(5~{S},6~{E},8~{S},9~{S},12~{R},15~{E})-21-chloranyl-12,20-dimethoxy-6,8,16-trimethyl-5,9-bis(oxidanyl)-2-azabicyclo[16.3.1]docosa-1(21),6,15,18(22),19-pentaene-3,11-dione 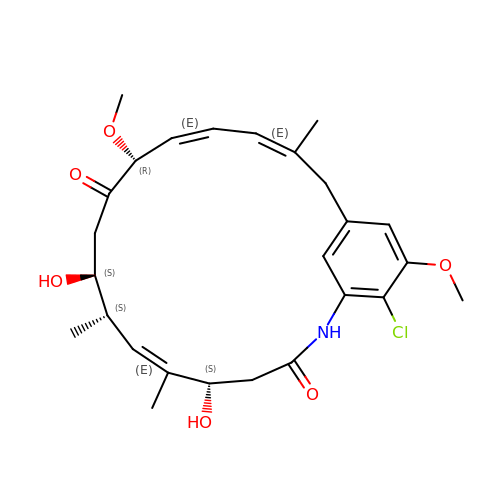| C26 H34 Cl N O6 | FDXIJEQRVYBNHT-SCFILQMVSA-N> GLPTMLTPGSNQFLTSDDFQSPSAMPQFDVTPEMKIPGEVHNLMEIAEVDSVVPVNNTKENINSMEAYRIPVTGGDQLHTQVFGFQ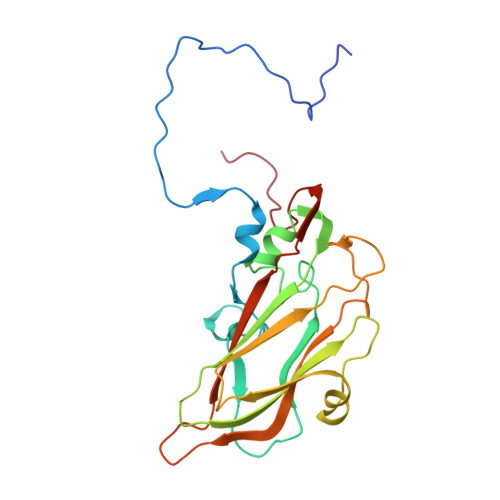MQPGLNSVFKRTLLGEILNYYAHWSGSVKLTFVFCGSAMATGKFLLAYSPPGASPPQNRKQAMLGTHVIWDVGLQSSCVLCIPWISQTHYRLVQQDEYTSAGYVTCWYQTGLIVPPGAPPSCTILCFASACNDFSVRNLRDTPFIEQTQLLQ>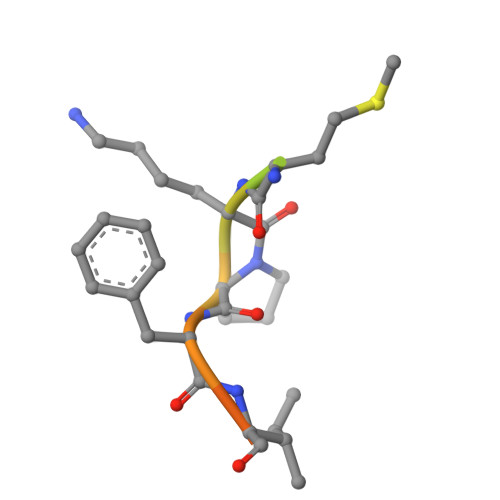 TRYANPKMKPFIFGAX> MEMAESVTNPQRPPVIWIGAQECTGCTESLLRATHPTVENLVLETISLEYHEV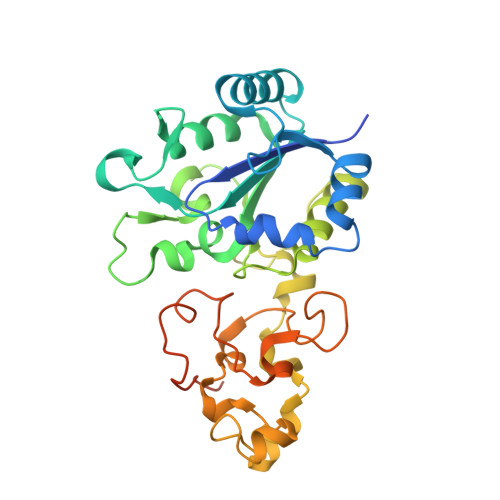LSAAFGHQVEENKHNALEKYKGQYVLVVDGSIPLKDNGIYCMVAGEPIVDHIRKAAEGAAAIIAIGSCSAWGGVAAAGVNPTGAVSLQEVLPGKTVINIPGCPPNPHNFLATVAHIITYGKPPKLDDKNRPTFAYGRLIHEHCERRPHFDAGRFAKEFGDEGHREGWCLYHLGCKGPETYGNCSTLQFCDVGGVWPVAIGHPCYGCNEEGIGFHKGIHQLANVENQTPRSQKPDVNAKEGGHHHHHH> IPCGESCVWGPCISSAIGCSCKSKVCYRNG;> IPCGESCVWLPCISSAIGCSCKSK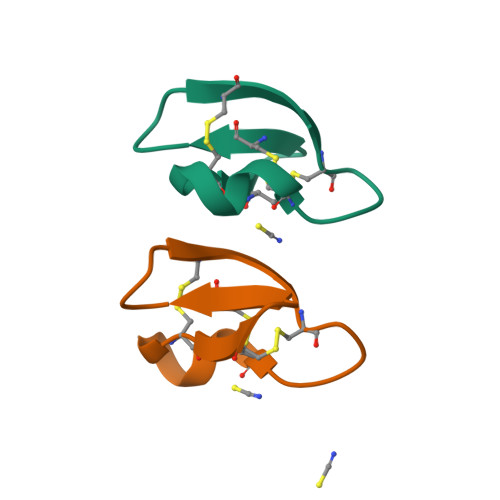VCYRNG> MGPVWRKHYITYRINNYTPDMNREDV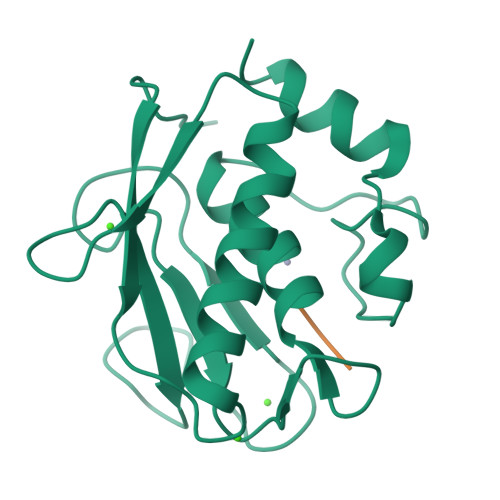DYAIRKAFQVWSNVTPLKFSKINTGMADILVVFARGAHGDDHAFDGKGGILAHAFGPGSGIGGDAHFDEDEFWTTHSGGTNLFLTAVHEIGHSLGLGHSSDPKAVMFPTYKYVDINTFRLSADDIRGIQSLYG;> IAG>VFQKAVDQSIEKKIVLRNGTEAFDSWEKPPLPVYTQFYFFNVTNPEEILRGETPRVEEVGPYTYRELRNKANIQFGDNGTTISAVSNKAYVFERDQSVGDPKIDLIRTLNIPVLTVIEWSQVHFLREIIEAMLKAYQQKLFVTHTVDELLWGYKDEILSLIHVFRPDISPYFGLFYEKNGTNDGDYVFLTGEDSYLNFTKIVEWNGKTSLDWWITDKCNMINGTDGDSFHPLITKDEVLYVFPSDFCRSVYITFSDYESVQGLPAFRYKVPAEILANTSDNAGFCIPEGNCLGSGVLNVSICKNGAPIIMSFPHFYQADERFVSAIEGMHPNQEDHETFVDINPLTGIILKAAKRFQINI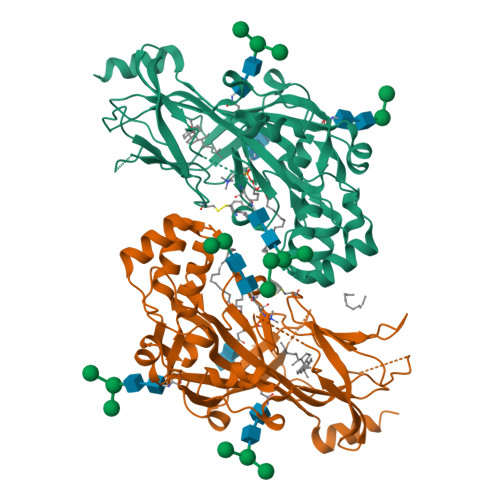YVKKLDDFVETGDIRTMVFPVMYLNESVHIDKETASRLKSMINTHHHHHH[2x]> GSSSRECSYCGKFFRSNYYLNIHLRTHTGEKPYKCEFCEYAA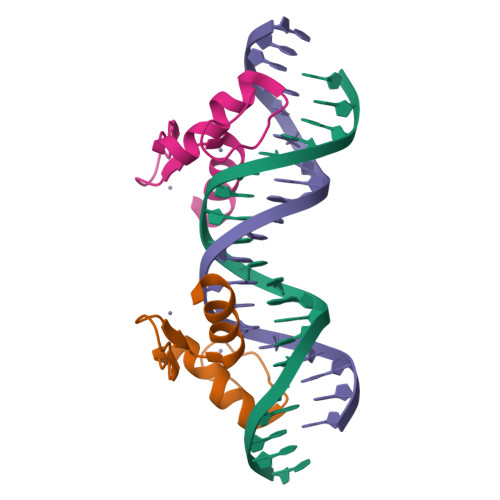AQKTSLRYHLERHHK> SNEKIRSQSVLNTLETFFIKENHYDMQREESSIVNACLRYLGY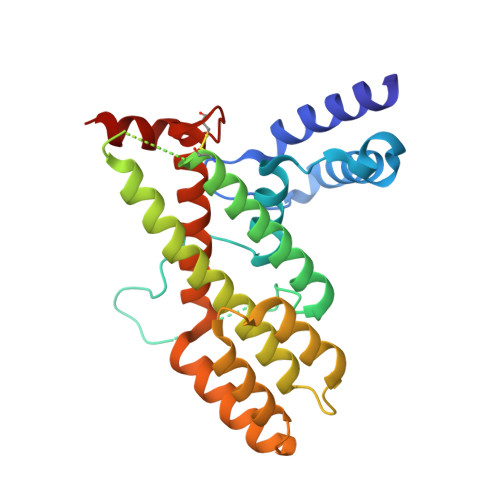SKSMCHEKMPIFMDIAFIEYCFNLSLDPSSFQNLPITQTQPDSQQILWEYSLISNALERLENIELERQNCMREDGLVKYTNELLLNKETLNNEALKLYSCAKAGICRWMAFHFLEQEPIDHINFTKFLQDWGSHNEKEMEALQRLSKHKIRKRLIYVSQHKKKMPWSKFNSVLSRYIQCTKLQLEVFCDYDFKQREIVKMLTSNIN KAT2A is the first identified histone acetyltransferase (HAT) and succinyltransferase. Here, we report that KAT2A can selectively utilize acetyl-CoA, propionyl-CoA, butyryl-CoA, and succinyl-CoA to directly deposit 18 histone acylation hallmarks in nucleosome. By analyzing the co-crystal structures of the catalytic domain of KAT2A in complex with acetyl-CoA, propionyl-CoA, butyryl-CoA, malonyl-CoA, succinyl-CoA, and glutaryl-CoA, we conclude that the alternative substrate-binding pocket of KAT2A and the length and electrostatic features of the acyl chain cooperatively determine the selection of the acyl-CoA substrates by KAT2A. Superimposition analyses revealed that all the studied acyl-CoA molecules fit in the same substrate-binding pocket, surrounded by the sheets of β4 and β6 and the helices of α3 and α5, indicating that all the studied acyl-CoA could potentially be utilized by KAT2A to modify histones.

Acetyl-CoA, propionyl-CoA, and butyryl-CoA are type I CoA molecules without a carboxyl group at the end of the acyl chains. As the acyl chain gets longer, the terminus extends to reach deeper into the binding pocket toward Loop 3, which might occupy the space for the incoming histone lysine residue. KAT2A has an alternative pocket for substrate binding. The propionyl and butyryl chain could flip into the alternative pocket, orienting the reactive carbonyl group of their acyl chain to receive proton transferred from the ε-amino group of the lysine substrate, allowing the covalent modification to occur. Thus, propionyl-CoA and butyryl-CoA can be utilized by KAT2A for histone modifications. By replacing the acyl-CoA with a hexanoyl-CoA model, we simulated the accommodation of hexanoyl-CoA which fits well in the KAT2A catalytic pocket, suggesting that KAT2A could potentially utilize acyl-CoAs with larger acyl chain than that of butyryl-CoA. The binding affinity of KAT2A to butyryl-CoA was unexpectedly affected by the Y645A mutation, indicating an additional interaction between the butyryl chain and the Tyr645 residue in KAT2A that was not noted previously. The interface analysis of the current structures showed a buried surface area of ~10 Å2 between Tyr645 and the butyryl chain, which is comparable to that between Tyr645 and the succinyl chain of ~7 Å2. Instead of the hydroxyl group that forms a hydrogen bond with the succinyl chain, it is the benzene ring of Tyr645 that is involved in the interaction with the butyryl chain.

>[8x]GIIEFHVIGNSLTPKANRRVLLWLVGLQNVFSHQLPRMPKEYIARLVFDPKHKTLALIKDGRVIGGICFRMFPTQGFTEIVFCAVTSNEQVKGYGTHLMNHLKEYHIKHNILYFLTYADEYAIGYFKKQGFSKDIKVPKSRYLGYIKDYEGATLMECELNPRIPYT>GSHMASFLKRYTSNTYSKDEEKLIQSVSKAVQYMAKRRIGALIVFEKETGLQDYIETGIAMDSNISQELLICVFIPNCPLHDGAMIIQGTKIAAAASYLPLSDSPKISKSLGTRHRAAVGISEVSDAF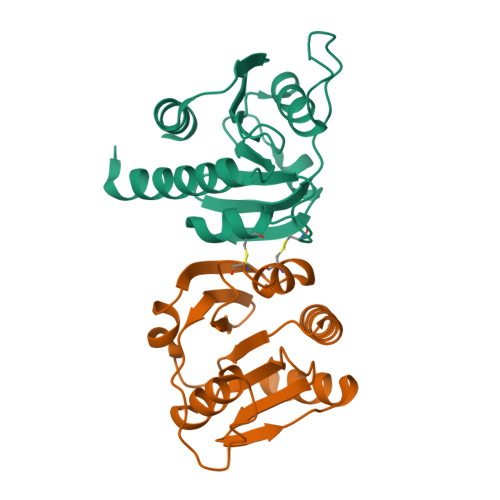TVIVSEETGDISVTFDGKLRRDISNEIFEELLAEHWFGTRFQKKGVK[2x]2-(2,5-dioxopyrrolidin-1-yl)acetamide 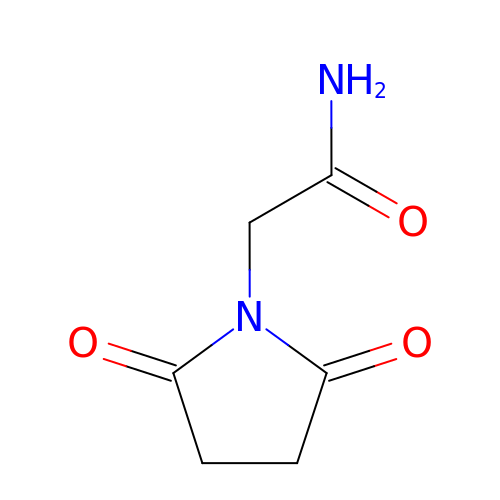| C6 H8 N2 O3 | RLSJGKULBJWLEW-UHFFFAOYSA-N> AASTT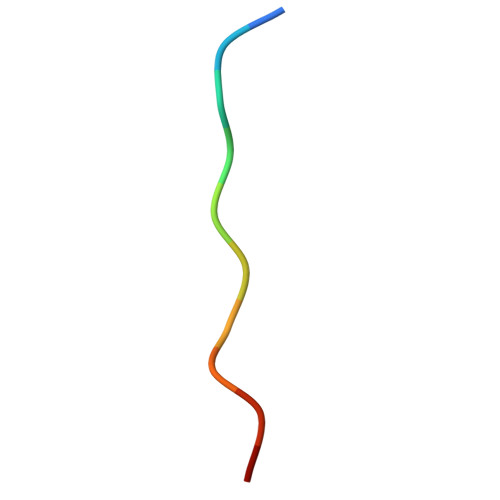TPAPAX> AAPGSVVELLGKSYPQDDHSNLTRKVLTRVGRNLHNQQHHPLWLIKERVKEHFYKQYVGRFGTPLFSVYDNLSPVVTTWQNFDSLLIPADHPSRKKGDNYYLNRTHMLRAHTSAHQWDLLHAGLDAFLVVGDVYRRDQIDSQHYPIFHQLEAVRLFSKHELFAGIKDGESLQLFEQSSRSAHKQETHTMEAVKLVEFDLKQMLTRLMAHLFGDELEIRWVDCYFPFTHPSFEMEINFHGEWLEVLGCGVMEQQLVN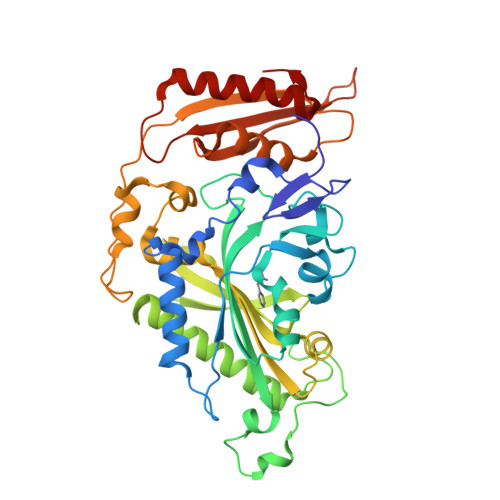SAGAQDRIGWAFGLGLERLAMILYDIPDIRLFWCEDERFLKQFCVSNINQKVKFQPLSKYPAVINDISFWLPSENYAENDFYDLVRTIGGDLVEKVDLIDKFVHPKTHKTSHCYRITYRHMERTLSQREVRHIHQALQEAAVQLLGVEGRF> RSKSSNEATNITPKHNMKAFLDELKAENIKKFLYNFTQIPHLAGTEQNFQLAKQIQSQWKEFGLDSVELAHYDVLLSYPNKTHPNYISIINEDGNEIFNTSLFEPPPPGYENVSDIVPPFSAFSPQGMPEGDLVYVNYARTEDFFKLERDMKINCSGKIVIARYGKVFRGNKVKNAQLAGAKGVILYSDPADYFAPGVKSYPDGWNLPGGGVQRGNILNLNGAGDPLTPGYPANEYAYRRGIAEAVGLPSIPVHPIGYYDAQKLLEKMGGSAPPDSSWRGSLKVPYNVGPGFTGNFSTQKVKMHIHSTNEVTRIYNVIGTLRGAVEPDRYVILGGHRDSWVFGGIDPQSGAAVVHEIVRSFGTLKKEGWRPRRTILFASWDAEEFGLLGSTEWAEENSRLLQERGVAYINADSSIEGNYTLRVDCTPLMYSLVHNLTKELKSPDEGFEGKSLYESWTKKSPSPEFSGMPRISKLGSGNDFEVFFQRLGIASGRARYTKNWETNKFSGYPLYHSVYETYELVEKFYDPMFKYHLTVAQVRGGMVFELANSIVQPFDCRDYAVVLRKYADKIYSISMKHPQEMKTYSVSFDSLFSAVKNFTEIASKFSERLQDFDKSNPIVLRMMNDQLMFLERAFIDPLGLPDRPFYRHVIYAPSSHNKYAGESFPGIYDALFDIESKVDPSKAWGEVKRQIYVAAF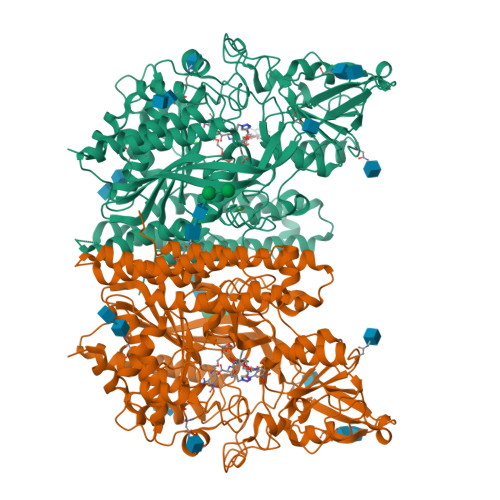TVQAAAETLSEVA> MKALVRLSSNHIFRSDSMSRVWLTGDAVVDLIPDGQQHYLKCPGGAPANVAVAIARLSGRSAFFGRVGNDPFGRFMQQTLTDEQVDCQHLHFDPVHRTSTVVVDLDECGERSFTFMVKPSADQFLQLSDIPSFQKGEWLHVCSIALANQPSRSSTFAAIAQMKEVGGYVSFDPNLREEVWSEPQELQATVMRAVGLADVVKFSEEELQFLTGTQSIEEGLQAIADFQIPLVVVTLGAKGALVATPNSQQIVSGKAVKPIDCTGAGDAFVGGLLYRLSVAQDWHNQATILDAVKWANGCGALATTQKGAMTALPNQAALYAFLE

Another fructokinase, FRK (EC 2.7.1.4), belongs to pfkB family of sugar kinase, catalyzes the phosphorylation of D-fructose to D-fructose-6-phosphate (F6P). V. cholerae FRK (VcFRK), encoded by cscK gene was predicted to have fructokinase activity according to KEGG pathway. Each monomer of VcFRK exhibits the typical ribokinase like fold consisting of a αβα three-layer sandwich domain and a lid domain. The flexible lid domain, which extends from the central β-sheet core, is formed by two pairs of antiparallel β-strands β2-β3 and β6-β7 and their connecting loops.

Upon fructose binding large lid domain of VcFRK moves towards αβα domain and traps the sugar. Crystal structure of VcFRK-fructose shows that H108 of the large lid domain and T261 of the αβα domain are very close, which were otherwise about 20 Å apart in the apo structure. To check the essentiality of loop closure and opening, in fructose binding and F6P release respectively, a double mutant H108C/T261C-VcFRK (henceforth designated as “VcFRK-DM”) was designed. Fructose bound VcFRK-DM structure (1.67 Å) shows that C108 and C261 are disulphide linked. Hence, VcFRK-DM is expected to remain in closed form upon fructose binding and thus unable to re-open during F6P release. Under reducing condition, VcFRK-DM exhibit comparable kinase activity compared to that of wild type VcFRK implying that H108C/T261C mutations do not hamper the kinase activity. The O6′ atom of fructose that would be phosphorylated remains accessible in both the VcFRK-DM-fructose and VcFRK-fructose structures. However, under mild oxidizing condition the rate of phosphotransfer reduces to nominal. Under oxidizing condition the disulfide bond formed between C108–C261, that tethers large lid domain with the αβα domain, would hinder the release of F6P from the active site. Therefore, our results suggest that closing and reopening of the lid during fructose binding or F6P release is essential for fructokinase activity.>MAHHHHHHMRLILLGAPGAGKGTQANFIKEKFGIPQISTGDMLRAAVKAGTPLGVEAKTYMDEGKLVPDSLIIGLVKERLKEADCANGYLFDGFPRTIAQADAMKEAGVAIDYVLEIDVPFSEIIERMSGRRTHPASGRTYHVKFNPPKVEGKDDVTGEPLVQRDDDKEETVKKRLDVYEAQTKPLITYYGDWARRGAENGLKAPAYRKISGLGAVEEIRARVRRAQVSE[2x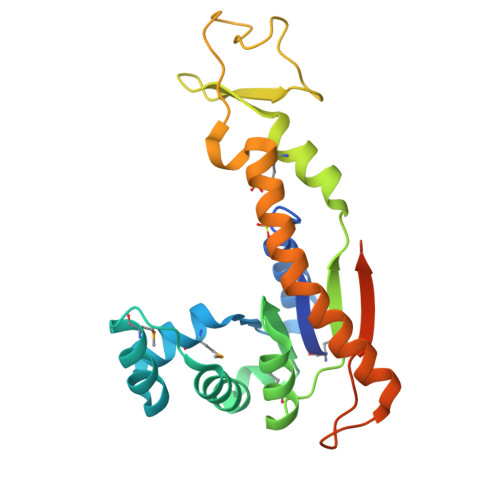]>[3x]MSLTTMLEVAKRAGVSKATVSRVLSGNGYVSQETKDRVFQAVEESGYRPNLLARNLSAKSTQTLGLVVTNTLYHGIYFSELLFHAARMAEEKGRQLLLADGKHSAEEERQAIQYLLDLRCDAIMIYPRFLSVDE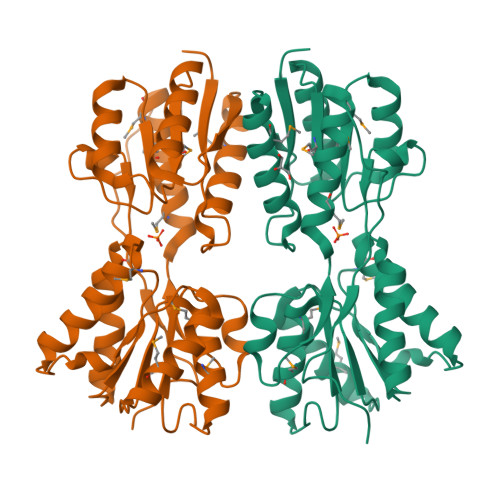IDDIIDAHSQPIMVLNRRLRKNSSHSVWCDHKQTSFNAVAELINAGHQEIAFLTGSMDSPTSIERLAGYKDALAQHGIALNEKLIANGKWTPASGAEGVEMLLERGAKFSALVASNDDMAIGAMKALHERGVAVPEQVSVIGFDDIAIAPYTVPALSSVKIPVTEMIQEIIGRLIFMLDGGDFSPPKTFSGKLIRRDSLIAPSR> QGPGGGGGSVTCPGGQSTSNSQCCVWFDVLDDLQTNFYQGSKCESPVRKILRIVFHDAIGFSPALTAAGQFGGGGADGSII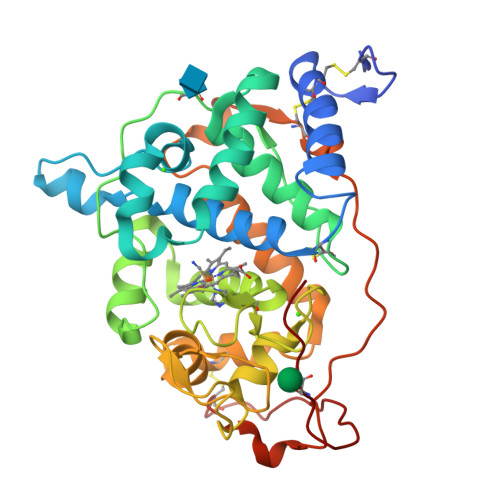AHSNIELAFPANGGLTDTIEALRAVGINHGVSFGDLIQFATAVGMSNCPGSPRLEFLTGRSNSSQPSPPSLIPGPGNTVTAILDRMGDAGFSPDEVVDLLAAHSLASQEGLNSAIFRSPLDSTPQVFDTQFYIETLLKGTTQPGPSLGFAEELSPFPGEFRMRSDALLARDSRTACRWQSMTSSNEVMGQRYRAAMAKMSVLGFDRNALTDCSDVIPSAVSNNAAPVIPGGLTVDDIEVSCPSEPFPEIATASGPLPSLAPAP>[12x]MTTLADVKKRIGLKDEKQDEQLEEIIKSCESQLLSMLPIEVEQIPERFSYMIKEVAVKRYNRIGAEGMTSEAVDGRSNAYELNDFKEYEAIIDNYFNARTRTKKGRAVFF;>[6x]MRYEDRVIFQLEQVATYNPKTSKKENTLITYDAIPCNINPISRARKQLEFGDVKNDVSVLRIKESISYPVSHVLVNGIRYKIVDTRIYRHETSYYIEEVN;>MTPNLQLYNKAYETLQGYGFPVISRKEMQQEIPYPFFVIKMPESNRSKYTFDSYSGDTNLVIDIWSVSDDLGHHDGLVKRCIDDLTPSVKTNDYDFEEDDTNITQLVDDTTNQELLHTSITISYKTF[6x];>[12x]MANMKNSNDRIILFRKAGEKVDATKMLFLTEYGLSHEADTDTEDTMDGSYNTGGSVESTMSGTAKMFYGDDFADEIEDAVVDRVLYEAWEVESRIPGKNGDSAKFKAKYFQGFHNKFELKAEANGIDEYEYEYGVNGRFQRGFATLPEAVTKKLKATGYRFHDTTKEDALTSEDLTAIPQPKVDSSTVTPGEV;>[3x]MTEYKIKATIEASVAKFKRQIDSAVKSVQRFKRVADQTKDVELNANDKKLQKTIKVAKKSLDAFSNKNVKAKLDASIQDLQQKILESNFELDKLNSKEASPEVKLQKQKLTKDIAEAENKLSELEKKRVNIDVNADNSKFNRVLKVSKASLEALNRSKAKAILDVDNSVANSKIKRTKEELKSIPNKTRSRLDVDTRLSIPTIYAF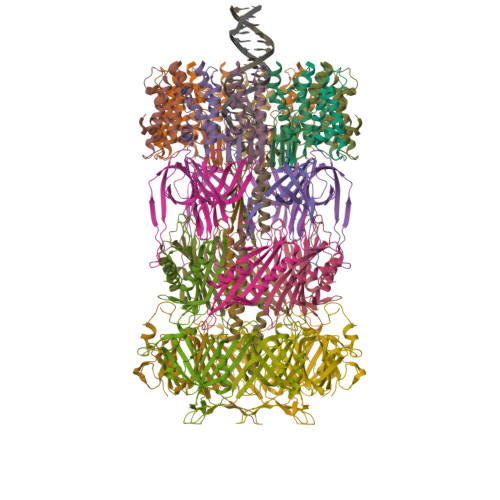KKSLDALPNKKTTKVDVDTNGLKKVYAYIIKANDNFQRQMGNLANMFRVFGTVGSNMVGGLLTSSFSILIPVIASVVPVVFALLNAIKVLTGGVLALGGAVAIAGAGFVAFGAMAISAIKMLNDGTLQASSATNEYKKALDGVKSAWTDIIKQNQSAIFTTLANGLNTVKTAMQSLQPFFSGISRGMEEASQSVLKWAENSSVASRFFNMMNTTGVSVFNKLLSAAGGFGDGLVNVFTQLAPLFQWSADWLDRLGQSFSNWANSAAGENSITRFIEYTKTNLPIIGNIFKNVFAGINNLMNAFSGSSTGIFQSLEQMTAKFREWSEQVGQSQGFKDFVSYIQTNGPLIMQLIGNIARGLVAFATAMAPIASAVLRVAVAITGWIANLFEAHPATAQLVGVIITLVGAFRFLIAPILAVMDFLGPLAARLVALVTKFGWAKTGTLVLSKAMTSLKGPIKLVTAIFQLLFGKIGLIRNAITGLVTVFGILGGPITIVIGVIAALIAIFVLLWNKNEGFRNFIINAWNAIKTFMVNVWNVLKAVASVVWNAILTAITTAVSNVYNFIMIVWNQIVAYLQGLWNGIIAIATTVWNLLVTIITTVFTTIMTIVMTIWTAIWTFLSTIWNTIITIATTIWNLLVTVITTVFTTIMTIAMTIWNAIWTFLQTLWNTIVTVATKVWNAITTAISTALQAAWSFISNIWNTIWSFLSGILTTIWNKVVSIFTQVVSTISDKMSQAWNFIVTKGMQWVSTITSTLINFVNRVIQGFVNVVNKVSQGMTNAVNKIKSFIGDFVSAGADMIRGLIRGIGQMAGQLVDAAKNVAKKALDAAKSALGIHSPSREFMDVGMYSMLGFVKGIDNHSSKVIRNVSNVADKVVDAFQPTLNAPDISSITGNLSNLGGNINAQVQHTHSIETSPNMKTVKVEFDVNNDALTSIVNGRNAKRNSEYYL;> MNIDGLDALLNQFHDMKTNIDDDVDDILQENAKEYVVRAKLKAREVMNKGYWTGNLSRNIRYKKTGDLQYTITSHAAYSGFLEFGTRYMEAEPFMWPVYEVIRKSTVEELKALFE The Tet(X) flavin-dependent monooxygenases enable tetracycline antibiotic resistance by catalysing inactivating hydroxylation, so preventing inhibition of bacterial ribosomes. Tetracycline destructases (TDases) are an emerging family of flavin-dependent monooxygenase (FMO) enzymes providing resistance to tetracyclines by catalysing C11a hydroxylation. C11a hydroxylation is proposed to hinder chelation of the tetracycline core to Mg2+ ions, thereby blocking binding to ribosomes and abolishing antibiotic activity. Importantly, Tet(X) enzymes, unlike their type 2 TDase counterparts, degrade third-generation tetracyclines, including tigecycline.

Prochlorperazine displayed improved activity compared to trifluoperazine, differing by replacement of the 2-trifluoromethyl-substituent with a chlorine, with an IC50app of 39.9 ± 7.0 and IC50 49.5 ± 24.9 μM in the FP- and UPLC-based assays, respectively. Clear electron density in the active site of Tet(X4) is observed for the tricyclic phenothiazine group in both the trifluoperazine and prochlorperazine complexes, including their 2-trifluoromethyl- and 2-chloro-substituents, respectively. The phenothiazine rings adopt near identical conformations (ESI Fig. S25†), suggesting a conserved binding mode. Analysis of the binding mode using Protein–Ligand Interaction Profiler (PLIP)63 reveals the phenothiazine groups make conserved hydrophobic contacts with residues Asn190, Gln192, Phe224 and Phe319. In the prochlorperazine complex and equivalent conformation with trifluoperazine, the protonated quaternary amine of the 4-methyl-piperazine group is proximal to Asp61 and Glu114 near the active site entrance, allowing for formation of a charge–charge interaction. Perazines, with a 3-(4-methylpiperazin-1-yl)propyl group attached to their 10-phenothiazinyl amine, bound with greater affinity than their promazine counterparts, which possess a N,N-dimethylpropan-1-amine group at the same position. The three compounds bind to the active site in a manner overlapping with the tigecycline binding site, validating their proposed mechanism of action as non-covalent competitive inhibitors. With all three compounds, the FAD cofactor appears in the so-called FAD-IN position (ESI Fig. S24†), wherein the catalytically-important isoalloxazine FAD ring is directed toward the tetracycline binding pocket, rather than the FAD-OUT conformation, where the isoalloxazine is instead directed towards the putative NADPH binding site.

> NLLSDKNVAIIGGGPVGLTMAKLLQQNGIDVSVYERDNDREARIFGGTLDLHKGSGQEAMKKAGLLQTYYDLALPMGVNIADEKGNILSTKNVKPENRFDNPEINRNDLRAILLNSLENDTVIWDRKLVMLEPGKKKWTLTFENKPSETADLVIIANGGMSKVRKFVTDTEVEETGTFNIQADIHHPEVNCPGFFQLCNGNRLMAAHQGNLLFANPNNNGALHFGISFKTPDEWKNQTQVDFQNRNSVVDFLLKEFSDWDERYKELIRVTSSFVGLATRIFPLGKSWKSKRPLPITMIGDAAHLMPPFAGQGVNSGLMDALILSDNLTNGKFNSIEEAIENYEQQMFIYGKEAQEESTQNEIEMFKPDFTF> NAKGNYCKRTPLYIDFKEIGWDSWIIAPPGYEAYECRGVCNYPLAEHLTPTKHAIIQALVHLKNSQKASKACCVPTKLEPISILYLDKGVVTYKFKYEGMAVSECGCR;> GSQNQERLCAFKDPYQQDLGIGESRISHENGTILCSKGSTCYGLWEKSKGDINLVKQGCWSHIGDPQECHYEECVVTTTPPSIQNGTYRFCCCSTDLCNVNFTENFPPPDTTPLSPPHSFNRDET

The TGF-β ligands are dimers and initiate signal transduction by forming a signalling complex with two copies of a type I receptor and two copies of a type II receptor; all are single-pass transmembrane proteins containing a small extracellular ligand-binding domain (ECD) and an intracellular kinase domain (ICD). Upon signalling complex formation, the constitutively active type II receptor phosphorylates and activates the type I receptor; subsequently the type I receptor phosphorylates Smad1/5 or Smad2/3 to regulate transcriptional responses. For example, ActRIIA/B bind to and mediate the signalling from both activin ligands and some BMP ligands, whereas BMPRII is the low-affinity type II receptor for over 15 BMP ligands. Of note, BMPRII is particularly highly expressed in lung vascular endothelial cells, where it mediates the signalling from circulating BMP9 and BMP10.

We solved crystal structures of the BMPRII binary complex with BMP10 in two different crystal forms, at 1.48 Å and 2.4 Å, respectively. In the 2.4 Å structure, there is only one copy each of BMP10 and BMPRII monomers in an asymmetric unit. The dimeric receptor complex can be generated with a symmetry-related molecule. Using the chain identities to name the seven complexes, they are complexes AC and BD, complex AB and complexes AI, BJ, CK and DL from the ternary complexes. Interestingly, 5 out of 15 residues with alternate conformations in complex AC are at this area, suggesting that the conformation in this region is highly flexible. Consistent with this observation, in complex BD and complex AB, the F3-loop region makes different interactions with BMP10 but both involve BMP10 residue D338 and are near BMPRII residue S107. Of note, these interactions are present in all three BMP10:BMPRII 1:1 complexes from the binary complexes, but not in those from the ternary complexes. S107 makes an additional interaction with BMP10 in binary complexes, but not in ternary complexes. In contrast, in the free ligand form, or in the complex with ALK1 (but no prodomain), BMP9 and 10 preferentially adopt the extended conformation. ENG-bound BMP9 is closer to the prodomain-bound form, whereas BMPRII-bound BMP10 (in the absence of ALK1) mostly adopts an intermediate conformation.> GAIEACLSAAGVPIDIPGTADYERDVEPFNIRLPYIPTAIAQTQTTAHIQSAVQCAKKLNLKVSAKSGGHSYASFGFGGENGHLMVQLDRMIDVISYNDKTGIAHVEPGARLGHLATVLNDKYGRAISHGTCPGVGISGHFAHGGFGFSSHMHGLAVDSVVGVTVVLADGRIVEASATENADLFWGIKGAGS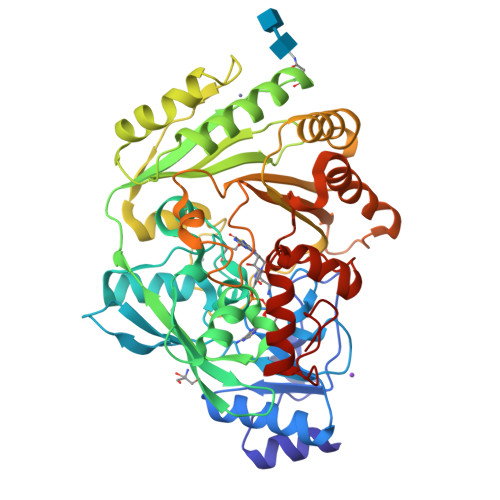NFGIVAVWKLATFPAPKVLTRFGVTLNWKNKTSALKGIEAVEDYARWVAPREVNFRIGDYGAGNPGIEGLYYGTPEQWRAAFQPLLDTLPAGYVVNPTTSLNWIESVLSYSNFDHVDFITPQPVENFYAKSLTLKSIKGDAVKNFVDYYFDVSNKVKDRFWFYQLDVHGGKNSQVTKVTNAETAYPHRDKLWLIQFYDRYDNNQTYPETSFKFLDGWVNSVTKALPKSDWGMYINYADPRMDRDYATKVYYGENLARLQKLKAKFDPTDRFYYPQAVRPVK>[2x]PFTMPKQTSGKYEKILQAAIEVISEKGLDKASISDIVKKAGTAQGTFYLYFSSKNALIPAIAENLLTHTLDQIKGRLHGDEDFWTVLDILID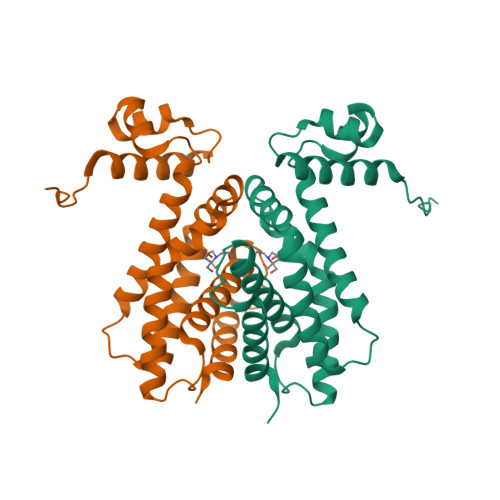ETFLITERHKDIIVLCYSGLAIDHSMEKWETIYQPYYSWLEKIINKAIANHEVTEGINSKWTARTIINLVENTAERFYIGFEQDENVEVYKKEIFTFLKRSLGTA2-[4-(3,5-dimethylpyrazol-1-yl)-2,6-bis(fluoranyl)phenyl]-~{N}-(4,5,6,7-tetrahydro-1,2-benzoxazol-3-yl)ethanamide 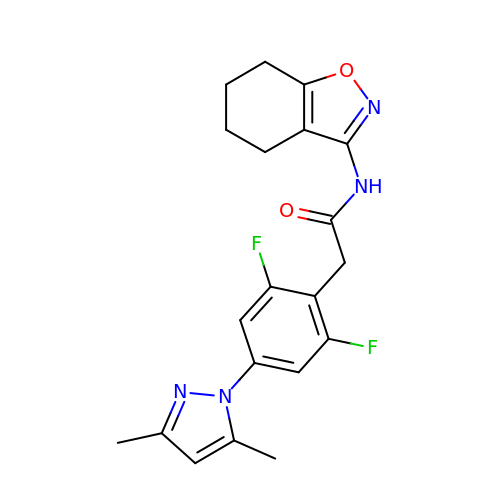| C20 H20 F2 N4 O2 | KHMWCMCBIAGTAK-UHFFFAOYSA-N> SELYRQSLEIISRYLREQATGAKDTKP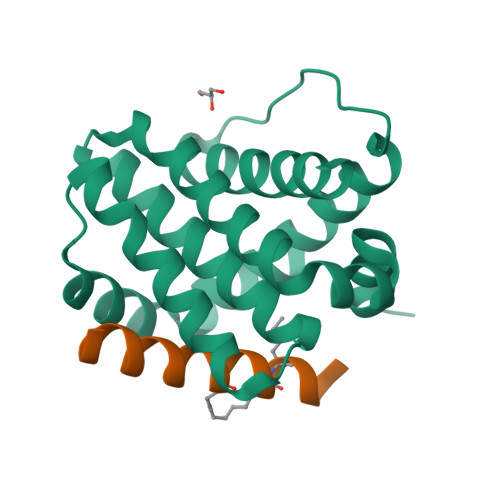MGRSGATSRKALETLRRVGDGVQRNHETAFQGMLRKLDIKNEDDVKSLSRVMIHVFSDGVTNWGRIVTLISFGAFVAKHLKTINQESCIEPLAESITDVLVRTKRDWLVKQRGWDGFVEFFHVEDLEGG;> XEDIIRNIARHLALVGDLLDRSIW>MEGGGKPNSSSNSRDDGNSVFPAKASATGAGPAAAEKRLGTPPGGGGAGAKEHGNSVCFKVDGGGGGGGGGGGGEEPAGGFEDAEGPRRQYGFMQRQFTSMLQPGVNKFSLRMFGSQKAVEKEQERVKTAGFWIIHPYSDFRFYWDLIMLIMMVGNLVIIPVGITFFTEQTTTPWIIFNVASDTVCLLDLIMNFRTGTVNEDSSEIILDPKVIKMNYLKSWFVVDFISSIPVDYIFLIVEKGMDSEVYKTARALRIVRFTKILCLLRLLRLSRLIRYIHQWEEIFHMTYDLASAVVRIFNLIGMMLLLAHWDGCLQFLVPLLQDFPPDCWVSLNEMVNDSWGKQYSYALFKAMSHMLCIGYGAQAPVSMSDLWITMLSMIVGATCYAMFVGHATALIQSLDSSRRQYQEKYKQVEQYMSFHKLPADMRQKIHDYYEHRYQGKIFDEENILNELNDPLREEIVNFNCRKLVATMPLFANADPNFVTAMLSKLRFEVFQPGDYIIREGAVGKKMYFIQHGVAGVITKSSKEMKLTDGSYFGEICLLTKGRRTASVRADTYCRLYSLSVDNFNEVLEEYPMMRRAFETVAIDRLDRIGKKNSILLQKFQKDLNTGVFNNQENEILKQIVKHDREMVQAIAPINYPQMTTL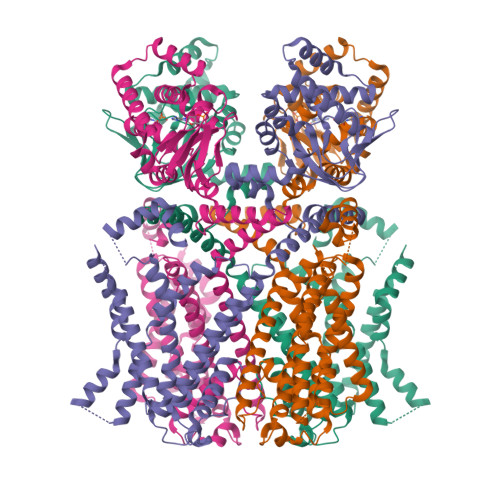NSTSSTTTPTSRMRTQSPPVYTATSLSHSNLHSPSPSTQTPQPSAILSPCSYTTAVCSPPVQSPLAARTFHYASPTASQLSLMQQQPQQQVQQSQPPQTQPQQPSPQPQTPGSSTPKNEVHKSTQALHNTNLTREVRPLSASQPSLPHEVSTLISRPHPTVGESLASIPQPVTAVPGTGLQAGGRSTVPQRVTLFRQMSSGAIPPNRGVPPAPPPPAAALPRESSSVLNTDPDAEKPRFASNL[4x]>[4x]ASVHGTTYELLRRQGIDTVFGNPGSNELPFLKDFPEDFRYILALQEACVVGIADGYAQASRKPAFINLHSAAGTGNAMGALSNAWNSHSPLIVTAGQQTRAMIGVEALLTNVDAANLPRPLVKWSYEPASAAEVPHAMSRAIHMASMAPQGPVYLSVPYDDWDKDADPQSHHLFDRHVSSSVRLNDQDLDILVKALNSASNPAIVLGPDVDAANANADCVMLAERLKAPVWVAPSAPRCPFPTRHPCF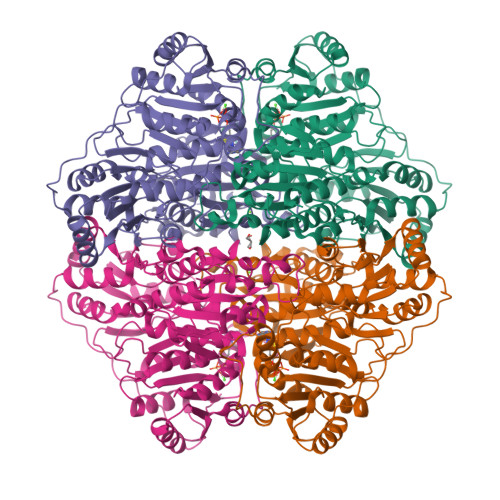RGLMPAGIAAISQLLEGHDVVLVIGAPVFRYAQYDPGQYLKPGTRLISVTCDPLEAARAPMGDAIVADIGAMASALANLVEESSRQLPTAAPEPAKVDQDAGRLHPETVFDTLNDMAPENAIYLNESTSTTAQMWQRLNMRNPGSYYFCAAGGLGFALPAAIGVQLAEPERQVIAVIGDGSANYSISALWTAAQYNIPTIFVIMNNGTYGALRWFAGVLEAENVPGLDVPGIDFRALAKGYGVQALKADNLEQLKGSLQEALSAKGPVLIEVSTVSPVKHHHHHH> HVKSGLQIKKNAIIDDYKVTSQVLGLGINGKVLQIFNKRTQEKFALKMLQDCPKARREVELHWRASQCPHIVRIVDVYENLYAGRKCLLIVMECLDGGELFSRIQDRGDQAFTEREASEIMKSIGEAIQYLHSINIAHRDVKPENLLYTSKRPNAILKLTDFGFAKETTSHNSLTEPCYTPYYVAPEV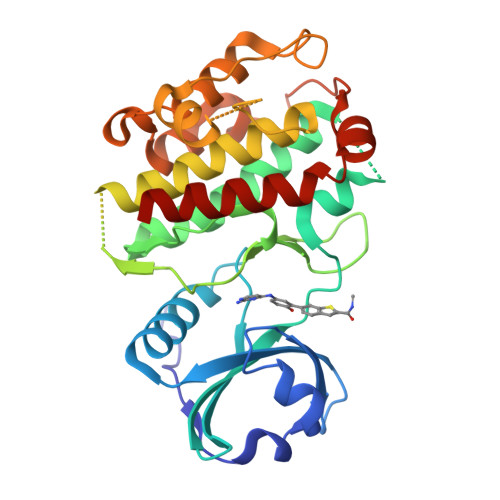LGPEKYDKSCDMWSLGVIMYILLCGYPPFYSNHGLAISPGMKTRIRMGQYEFPNPEWSEVSEEVKMLIRNLLKTEPTQRMTITEFMNHPWIMQSTKVPQTPLHTSRVLKEDKERWEDVKEEMTSALATMRVD> MESGDEAAIERHRVHLRSATLRDAVPATLHLLPCEVAVDGPAPVGRFFTPAIRQGPEGLEVSFRGRCLRGEEVAVPPGLVGYVMVTEEKKVSMGKPDPLRDSGTDDQEEEPLERDFDRFIGATANFSRFTL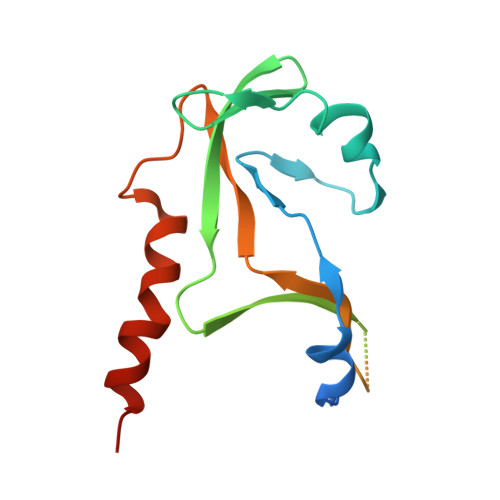WGLETIPGPDAKVRGALTWPSLAAAIHAQVPED> XRYAVVP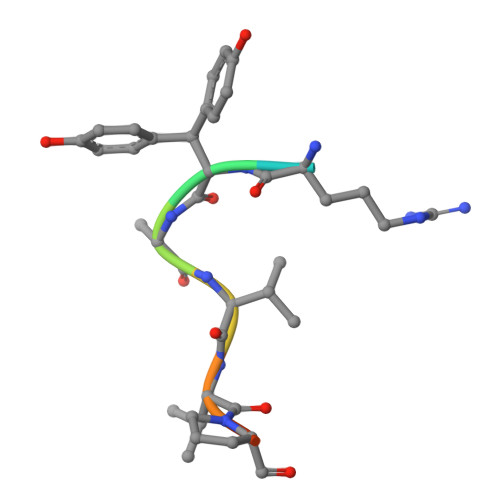DE>MGSSHHHHHHS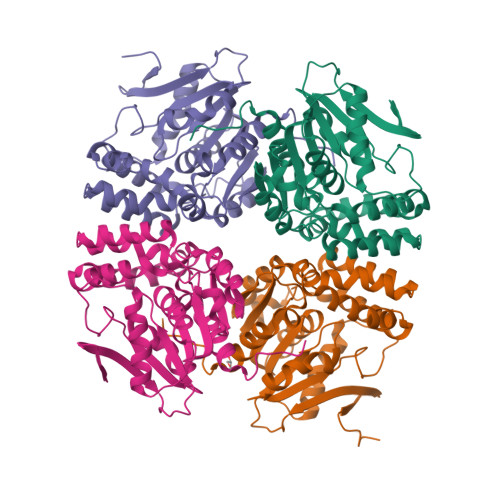SGRENLYFQGVSIFTYQEKDIYYEIDGTLDINSDVIVILNGIMMSTKSWDAFVENFSKNHVLLRYDMFDQGQSSKIEESYTQTIQVELLKNLLEHLGIAQANIVGISYGASIALQFAAKYPTMIKRMVVANVVAKTSPWLKDIGDGWNEVAKTGNGLAYYHITIPYIYSPQFYTLHNDWMEKRKELLVPLFSTRTFLDRMIRLTKSAETHDVIKDLPNIKTPTLIISSEEDYLTPPFEQKYLQEHLQNAELVSIPNCGHASMYEVPKTFTALVLGFFGQTKLDYQI[8x]>[2x]MNPIAVTLLTGFLGAGKTTLLRHILNEQHGYKIAVIENEFGEVSVDDQLIGDRATQIKTLTNGCICCSRSNELEDALLDLLDNLDKGNIQFDRLVIECTGMADPGPIIQTFFSHEVLCQRYLLDGVIALVDAVHADEQMNQFTIAQSQVGYADRILLTKTDVAGEAEKLHERLARINARAPVYTVTHGDIDLGLLFNTNGFMLEENVVSTKPRFHFIADKQNDISSIVVELDYPVDISE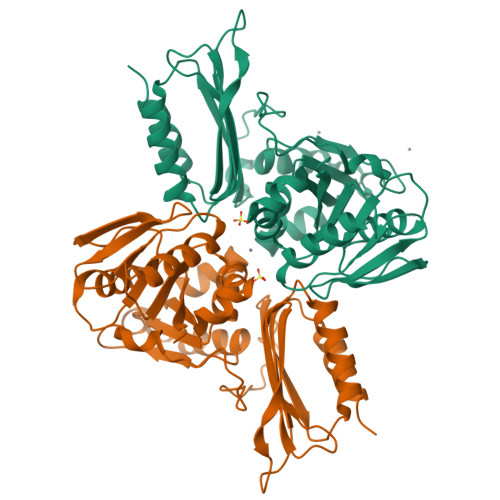VSRVMENLLLESADKLLRYKGMLWIDGEPNRLLFQGVQRLYSADWDRPWGDEKPHSTMVFIGIQLPEEEIRAAFAGLRK> MLIQAVGVNLPPSYVCLEGPLGGERPRAQGDEMLMQRLLPAVREALDEAAVKPEEIDLIVGLALSPDHLIENRDIMAPKIGHPLQKVLGANRAHVFDLTDSSLARALYVVDTLASDQGYRNVLVVRGESSQGLEVDSESGFALADGALALLCRPTGKAAFRRGALGGDPAQEWLPLSIPLNTDIRQVGDVKGHLNLPAQPGLPEAVRAGFTRLAGDFPQLNWVREEWFGQGRPDGRCLGPFELASQLRAAQRDRLDELLLISFDPFGM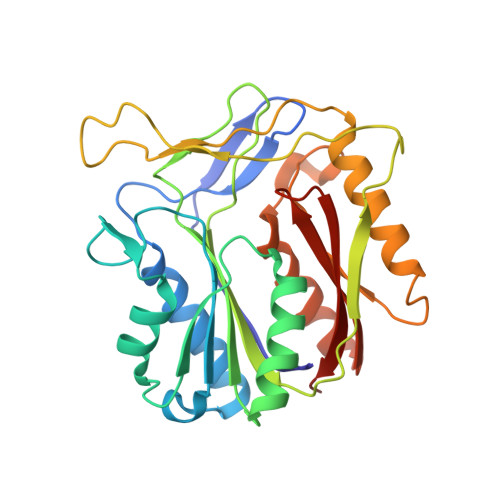VVEGVTLELAGEAHA> ASMTGGQQMGAPITAYAQQTRGLLGCIITSLTGRDKNQVEGEVQIVSTATQTFLATCINGVCWTVYHGAGTRTIASPKGPVIQMYTNVDQDLVGWPAPQGSRSLTPCTCGSSDLYLVTRHADVIPVRRRGDSRGSLLSPRPISYLKGSSGGPLLCPAGHAVGLFRAAVCTRGVTKAVDFIPVENLET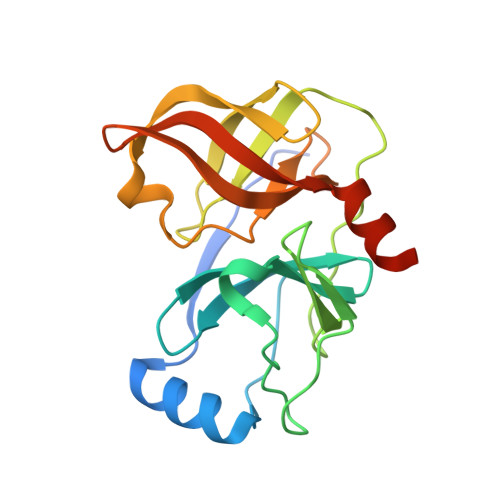TMRGSHHHHHH>[14x]NLIPTVIEQTNRGERAYD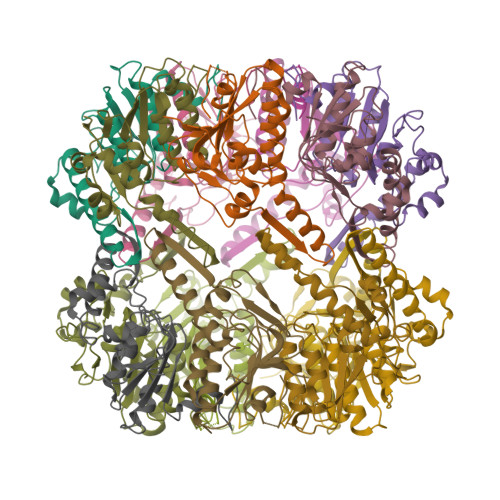IYSRLLKDRIIMLGSAIDDNVANSIVSQLLFLAAEDPEKEISLYINSPGGSITAGMAIYDTMQFIKPKVSTICIGMAASMGAFLLAAGEKGKRYALPNSEVMIHQPLGGAQGQATEIEIAAKRILLLRDKLNKVLAERTGQPLEVIERDTDRDNFKSAEEALEYGLIDKILTHTEDKKHHHHHH> MAENTKNENITNILTQKLIDTRTVL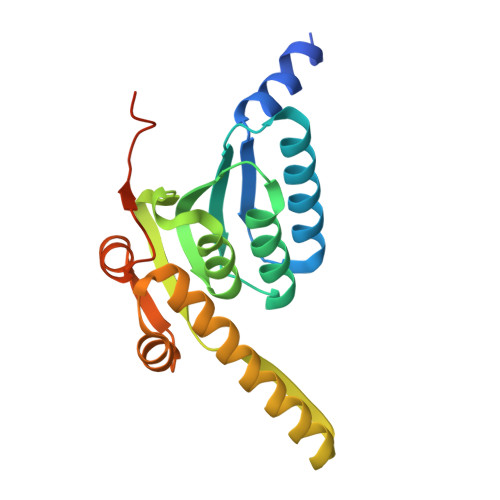IYGEINQELAEDVSKQLLLLESISNDPITIFINSQGGHVEAGDTIHDMIKFIKPTVKVVGTGWVASAGITIYLAAEKENRFSLPNTRYMIHQPAGGVQGQSTEIEIEAKEIIRMRERINRLIAEATGQSYEQISKDTDRNFWLSVNEAKDYGIVNEIIENRDGLKMASWSHPQFEK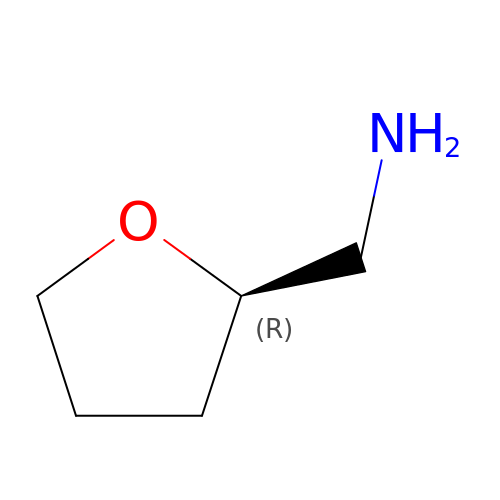1-[(2R)-oxolan-2-yl]methanamine | C5 H11 N O | YNOGYQAEJGADFJ-UHFFFAOYSA-N> GSPPEIKPFYFSSSVQEGQREQVICSAITGDLPLLFSWKKDGLIVE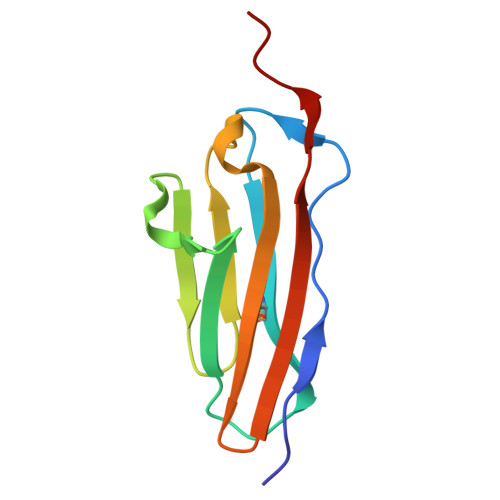NFKDITLVTNDLFSVLVISSIKPEHIGNYTCNLENPFGSDVHTAALTMKVPELS>[2x]MDFKYTEEKETIKINNIMIAKYTVLYTSNCIMDIYSEEEKITCFSNRLVFLERGVNISVRMQKQILSEKPYVAFRLNGDMLRHLKDALMIIYGMSKIDTNACRSMSRKIMTTEVNKTLLDELKNINSHDNSAFISSLIYLISKLENNEKIIESIYISSVSFFSDKVRNLIEKDLSRKWTLGIIADAFNASEITIRKRLESENTNFNQILMQLRMSKAALLLLENSYQISQISN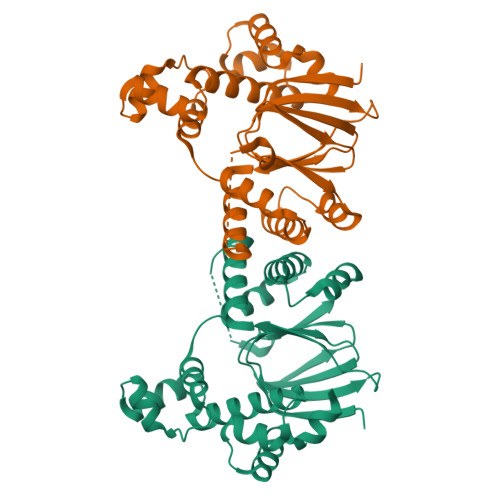MIGISSASYFIRIFNKHYGVTPKQFFTYFKGG> MTDTATTPQTTDAPAFPSNRSCPYQLPDGYAQLRDTPGPLHRVTLYDGRQAWVVTKHEAARKLLGDPRLSSNATDDNFPATSPAFEAVRESPQAFIGLDPPEHGTRRRMTISEFTVKRIKGMRPEVEEVVHGFLDEMLAAGPTADLVSQFALPVPSMVICRLLGVPYADHEFFQDASKRLVQSTDAQSALTARNDLAGYLDGLITQF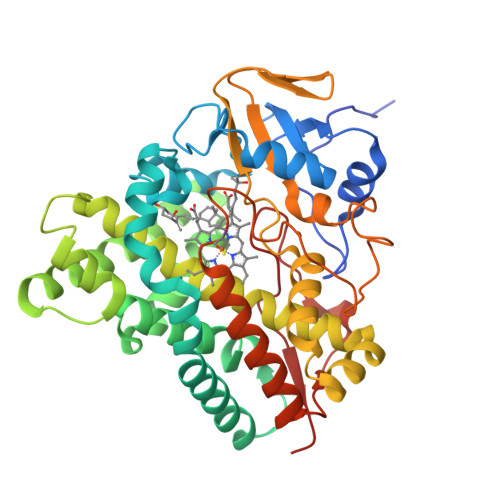QTEPGAGLVGALVADQLANGEIDREELISTAMLLLIAGHETTASMTSLSVITLLDHPEQYAALRADRSLVPGAVEELLRYLAIADIAGGRVATADIEVEGQLIRAGEGVIVVNSIANRDGTVYEDPDALDIHRSARHHLAFGFGVHQCLGQNLARLELEVILNALMDRVPTLRLAVPVEQLVLRPGTTIQGVNELPVTWHHHHHH>MAGSKVDKTLCRLGDITGLLIVLSVLVSRGLCQDCNNTNASSMADEKRLLKCILHDYDTAIRPVQNVSDVVNVALEVTVVKVIDLDEKEHVLTTNGWIYHEWNDFQLKWNPSDYSGLKKIRIPVDRIWTPDIVLFNNADESYRYVVDKLAVVYYTGKVMWVPHARLRSFCVLDLSRFPFDSQMCTLVFGSWTHDVSSVNVTLRNQSKVQYMIDGKEWQVTSVQPKRYQWTYNSNENYAGIITGIKLKRTSIYYQYVFIMPTVLLAFLTLLMPFIPPLGKERITYGIGLVLGCTLLLMMLSDRMPTELGNVPVVAAYLAYVFVMVAINLLFAIMAINMSMRDPKFGKVPGWVRWIFLTKLSKLVCLPVEPYTAVPADLAYEETAAARELLDMNNGTATADQRVSGSDTKPALDRTLEDIRRYLRLVATRTVVTPQLSHRDLVVQEWQQLTRVIDRLLFGSFLVLTVVITISMYAHY[5x]

Cys-loop receptors are allosterically regulated pentameric ligand-gated ion channels (pLGICs). In this work, we studied orphan receptor Alpo4 from an extreme thermophile worm Alvinella pompejana. Each Alpo4 subunit is composed of a β-sandwich extracellular domain (ECD) and a transmembrane domain (TMD) made of four trans-membrane α-helices M1-M4. In conclusion, Alpo4 has a pore structure consistent with a cation-selective channel, but with an unusually tight constriction at the 16’M position, the role of which remains unclear.

Either CHAPS was removed from the Alpo4CHAPS using size exclusion chromatography or we purified Alpo4 without any CHAPS present. Similar results were obtained from the sample prepared in LMNG without CHAPS, reconstructed to 4.1 Å. This structure is essentially identical to the apo state with (RMSD of 0.9 Å). No residual density was observed in the ligand-binding pocket in the later reconstruction, supporting the assignment of the 3.4 Å map as an apo state. The unmasked reconstruction (red) reaches 4.9 Å while the tight dynamic masked reconstruction (blue) reaches 4.1 Å.2-[2-[[3-(1,2,3,4-tetrahydroisoquinolin-7-yl)phenyl]methoxy]phenyl]ethanoic acid | C24 H23 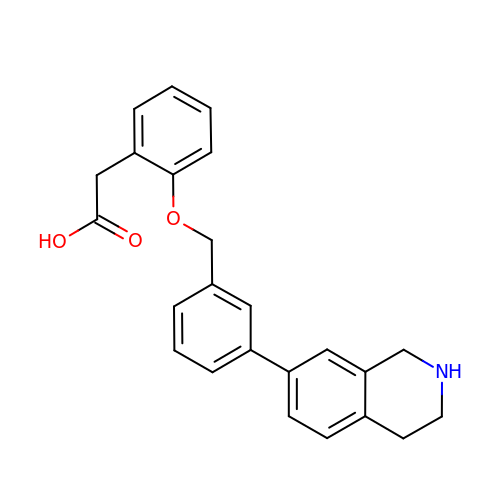N O3 | PKSHGMOAJDEGBL-UHFFFAOYSA-N>MGSSHHHHHHSQASIFVATSFWAALGNAGDARHGTAKRLWASKPPVVMTSNHVLGETWTLLNR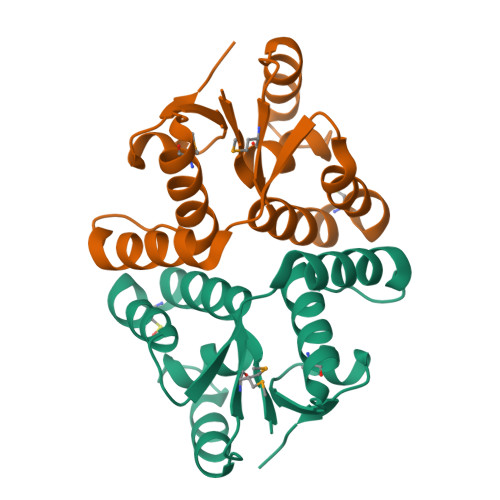RCGHRAAVAAAAIRLSTVVRVEHVTADLEEQAWEWLVRHDEREYSFVDATSFAVMRKKGIQNAYAFDGDFSAAGFVEVRPE[2x]> AEQSSSEIKIVRDEYGMPHIYANDTWHLFYGYGYVVAQDRLFQMEMARRSTQGTVAEVLGKDFVKFDKDIRRNYWPDAIRAQIAALSPEDMSILQGYADGMNAWIDKVNTNPETLLPKQFNTFGFTPKRWEPFDVAMIFVGTMANRYSDSTSEIDNLALLTALKDKYGVSQGMAVFNQLKWLVNPSAPTTIAVQESNYPLKFNQQNSQT;> SNMWVIGKSKAQDAKAIMVNGPQFGWYAPAYTYGIGLHGAGYDVTGNTPFAYPGLVFGHNGVISWGSTAGFGDDVDIFAERLSAEKPGYYLHNGKWVKMLSREETITVKNGQAETFTVWRTVHGNILQTDQTTQTAYAKSRAWDGKELASLLAWTHQMKAKNWQEWTQQAAKQALTINWYYADVNGNIGYVHTGAYPDRQSGHDPRLPVPGTGKWDWKGLLPFEMNPKVYNPQSGYIANWNNSPQKDYPASDLFAFLWGGADRVTEIDRLLEQKPRLTADQAWDVIRQTSRQDLNLRLFLPTLQAATSGLTQSDPRRQLVETLTRWDGINLLNDDGKTWQQPGSAILNVWLTSMLKRTVVAAVPMPFDK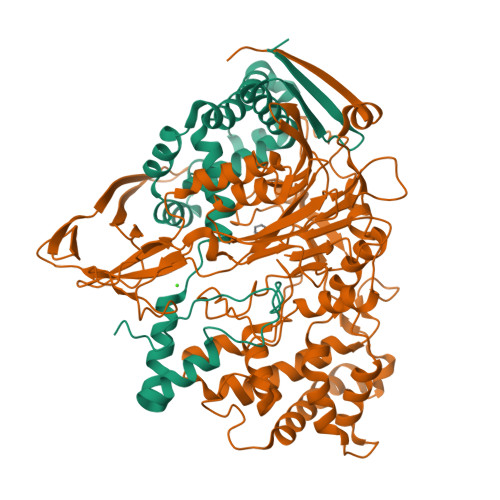WYSASGYETTQDGPTGSLNISVGAKILYEAVQGDKSPIPQAVDLFAGKPQQEVVLAALEDTWETLSKRYGNNVSNWKTPAMALTFRANNFFGVPQAAAEETRHQAEYQNRGTENDMIVFSPTTSDRPVLAWDVVAPGQSGFIAPDGTVDKHYEDQLKMYENFGRKSLWLTKQDVEAHKESQEVLHVQR(3E)-4-(2,6,6-trimethylcyclohex-1-en-1-yl)but-3-en-2-one 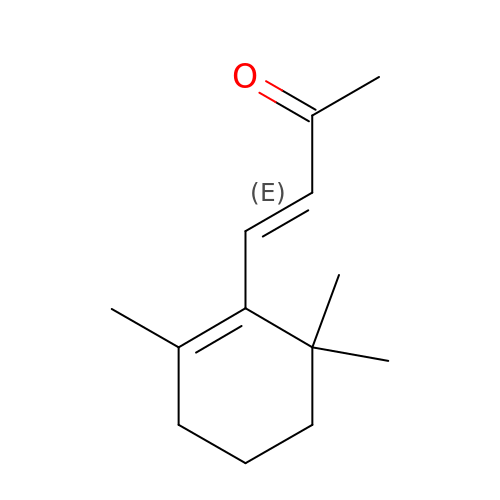| C13 H20 O | PSQYTAPXSHCGMF-BQYQJAHWSA-N> GKAFDDGAFTGIREINLSYNKETAIGDFQVVYDL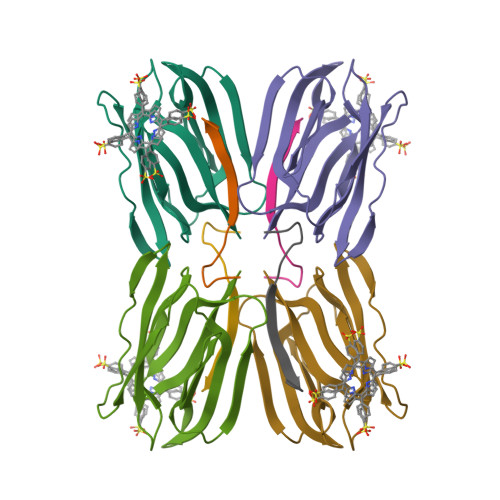NGSPYVGQNHKSFITGFTPVKISLDFPSEYIMEVSGYTGNVSGYVVVRSLTFKTNKKTYGPYGVTSGTPFNLPIENGLIVGFKGSIGYWLDYFSMYLSL;> DEQSGISQTVIVGPWGAKVS> GTGAMWLTKLVLNPASRAARRDLANPYEMHRTLSKAVSRALEEGRE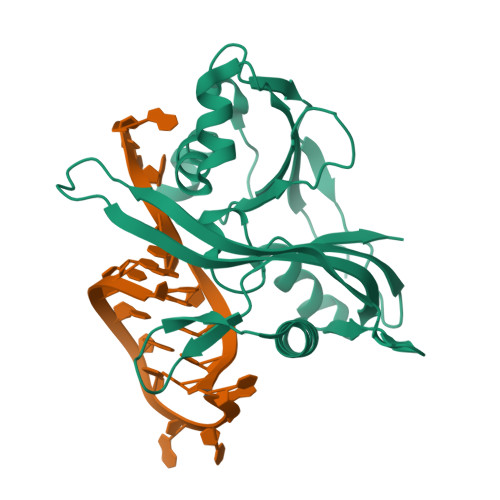RLLWRLEPARGLEPPVVLVQTLTEPDWSVLDEGYAQVFPPKPFHPALKPGQRLRFRLRANPAKRLAATGKRVALKTPAEKVAWLERRLEEGGFRLLEGERGPWVQILQDTFLEVRRKKDGEEAGKLLQVQAVLFEGRLEVVDPERALATLRRGVGPGKALGLGLLSVAP The plant satellite virus, satellite tobacco necrosis virus (STNV), is one such model. It is an example of a T = 1 capsid and is one of the smallest known viruses with a diameter of only 17 nm. A great deal is known about the virion structure and it was only the third virus to have its structure determined at atomic resolution. Its CP subunit has a Swiss-roll topology similar to that seen for the first two virus structures determined (tomato bushy stunt virus and southern bean mosaic virus)4,18–20 and now known to be present in the CPs of Picornaviridae. The N-terminal region of the protein is positively charged and forms an arm that is a common feature of many plant viruses, which is believed to interact non-sequence specifically with the viral RNA.

We were also able to use SELEX to isolate a preferred RNA binding motif for the CP. This is a short stem–loop structure with a loop sequence of AXXA, presented in 4-, 5-, or 6-base loops. The VLP reassembled in the presence of B3 crystallised, and its X-ray structure at 2.3 Å resolution was determined. The biggest difference between the B3 VLP structure and previously determined ones is that here the N-terminus is more ordered, permitting the formation of an additional turn at the N-terminus of the helix (residues 8–11 RKSA). Since the helices sit at 3-fold axes in the virion, this sequence-specific RNA–CP interaction has resulted in at least six positively charged residues coming into proximity. This may account for the inability of the CP to self-assemble in the absence of RNA and suggests that the capsomere may be a protein trimer. There is strong electron density for the B3 RNA that encompasses the smaller region of RNA density observed in the mRNA VLP. There is also significant additional density along the particle 2-fold axes adjacent to the tips of the N-terminal helices. As the RNA density in the B3 complex is not well defined, we have not attempted to model its interactions with the capsid. Some of the RNA binding sites must therefore be unoccupied.

> MAKQQNNRRKSATMRAVKRMINTHLEHKRFALINSGNTNATAGTVQNLSNGIIQGDDINQRSGDQVRIVSHKLHVRGTAITVSQTFRFIWFRDNMNRGTTPTVLEVLNTANFMSQYNPITLQQKRFTILKDVTLNCSLTGESIKDRIINLPGQLVNYNGATAVAASNGPGAIFMLQIGDSLVGLWDSSYEAVYTDA> MGSSHHHHHHSSGREALYFMGHMILVYSTFPNEEKALEIGRKLLEKRLI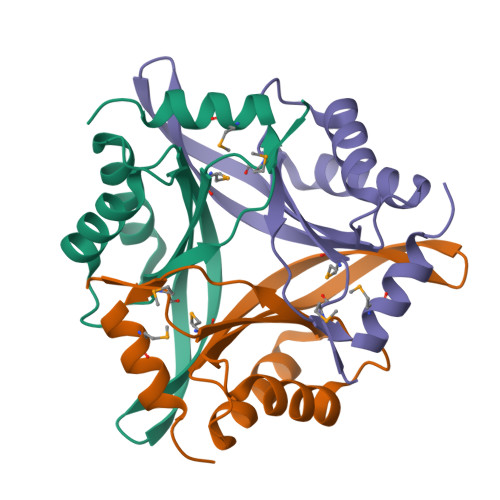ACFNAFEIRSGYWWKGEIVQDKEWAAIFKTTEEKEKELYEELRKLHPYETPAIFTLKVENILTEYMNWLRESVLGS PENTABROMOPSEUDILIN | C10 H4 Br5 N O | 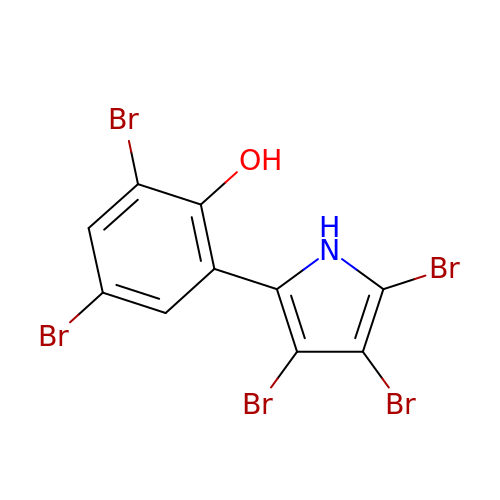LXMNWKJHYOZUQL-UHFFFAOYSA-N>[20x]SLINTKIKPFKNQAFKNGEFIEVTEKDTEGRWSVFFFYPADFTFV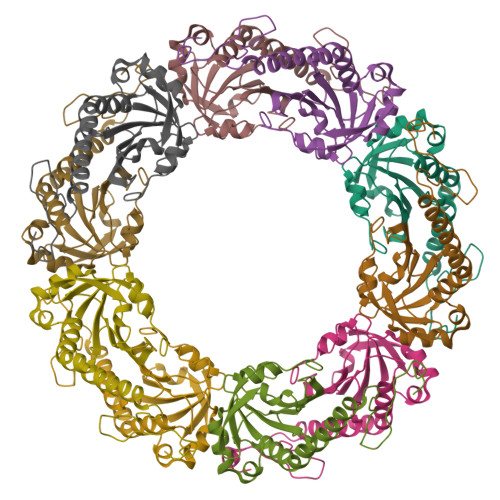SPTELGDVADHYEELQKLGVDVYSVSTDTHFTHKAWHSSSETIAKIKYAMIGDPTGALTRNFDNMREDEGLADRATFVVDPQGIIQAIEVTAEGIGRDASDLLRKIKAAQYVAAHPGEVCPAKWKEGEATLAPSLDLVGKI>[2x]MLQELPTLTPGQYSLVFNMFSFTVATMTASFVFFVLARNNVAPKYRISMMVSALVVFIAGYHYFRITSSWEAAYALQNGMYQPTGELFNDAYRYVD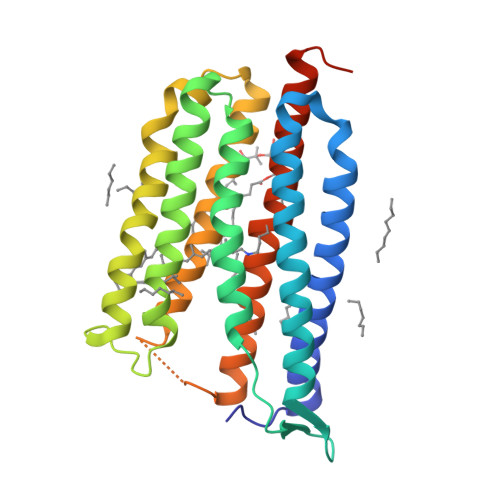WLLTVPLLTVELVLVMGLPKNERGPLAAKLGFLAALMIVLGYPGEVSENAALFGTRGLWGFLSTIPFVWILYILFTQLGDTIQRQSSRVSTLLGNARLLLLATWGFYPIAYMIPMAFPEAFPSNTPGTIVALQVGYTIADVLAKAGYGVLIYNIAKAKSEEEGFNVSEMVEPATASA>MKGFAMLSIGKVGWIEKEKPAPGPFDAIVRPLAVAPCTSDIHTVFEGAIGERHNMILGHEAVGEVVEVGSEVKDFKPGDRVVVPAITPDWRTSEVQRGYHQHSGGMLAGWKFSNVKDGVFGEFFHVNDADMNLAHLPKEIPLEAAVMIPDMMTTGFHGAELANIKLGDTVCVIGIG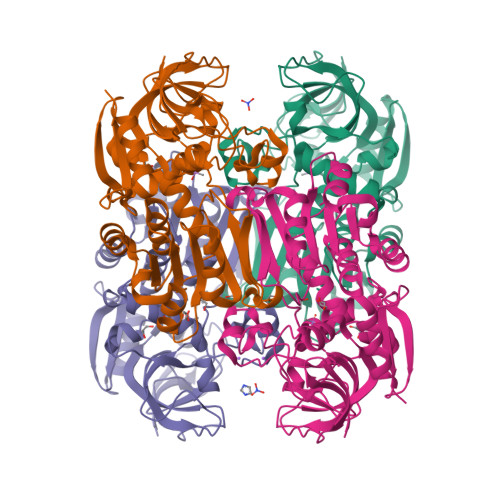PVGLMSVAGANHLGAGRIFAVGSRKHCCDIALEYGATDIINYKNGDIVEQILKATDGKGVDKVVIAGGDVHTFAQAVKMIKPGSDIGNVNYLGEGDNIDIPRSEWGVGMGHKHIHGGLCPGGRLRMERLIDLVFYKRVDPSKLVTHVFRGFDNIEKAFMLMKDKPKDLIKPVVILA[4x]> MKKEVRKVRIALASPEKIRSWSYGEVEKPETINYRTLKPERDGLFDERIFGPIKDYECACGKYKRQRFEGKVCERCGVEVTRSIVRRYRMGHIELATPAAHIWFVKDVPSKIGTLLDLSATELEQVLYFNKYIVLDPKGAVLDGVPVEKRQLLTDEEYRELRYGKQETYPLPAGVDALVKDGEEVVKGQELAPGVVSRMDGVALYRFPRRVRVDYLRKERAALRIPLSAWVEKEAYRPGEVLAELSEPYLFRAEESGVVELKDLAEGHLIYLRQEEEVVARYFLPAGMTPLVVEGEIVEVGQPLAEGKGLLRLPRHMTAKEVEAEEEGDSVHLTLFLEWTEPKDYKVAPHMNVIVPEGAKVQAGEKIVAAIDPEEEVIAEAEGVVHLHEPASILVVKARVYPFEDDVEVTTGDRVAPGDVLADGGKVKSEIYGRVEVDLVRNVVRVVESYDIDARMGAEAIQELLKELDLEKLERELLEEMKHPSRARRAKARKRLEVVRAFLDSGNRPEWMILEAVPVLPPDLRPMVQVDGGRFATSDLNDLYRRLINRNNRLKKLLAQGAPEIIIRNEKRMLQEAVDAVIDNGRRGSPVTNPGSERPLRSLTDILSGKQGRFRQNLLGKRVDYSGRSVIVVGPQLKLHQCGLPKRMALELFKPFLLKKMEEKAIAPNVKAARRMLERQRDIKDEVWDALEEVIHGKVVLLNRAPTLHRLGIQAFQPVLVEGQSIQLHPLVCEAFNADFDGDQMAVHVPLSSFAQAEARIQMLSAHNLLSPASGEPLAKPSRDIILGLYYITQVRKEKKGAGMAFATPEEALAAYERGEVALNAPIVVAGRETSVGRLKFVFANPDEALLAVAHGLLDLQDVVTVRYLGRRLETSPGRILFARIVGEAVGDEKVAQELIQMDVPQEKNSLKDLVYQAFLRLGMEKTARLLDALKYYGFTLSTTSGITIGIDDAVIPEEKQRYLEEADRKLRQIEQAYEMGFLTD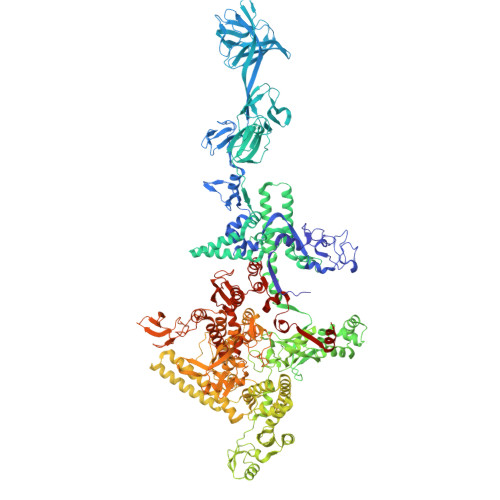RERYDQVIQLWTETTEKVTQAVFKNFEENYPFNPLYVMAQSGARGNPQQIRQLCGMRGLMQKPSGETFEVPVRSSFREGLTVLEYFISSHGARKGGADTALRTADSGYLTRKLVDVAHEIVVREADCGTTNYISVPLFQMDEVTRTLRLRKRSDIESGLYGRVLAREVEALGRRLEEGRYLSLEDVHFLIKAAEAGEVREVPVRSPLTCQTRYGVCQKCYGYDLSMARPVSIGEAVGVVAAESIGEPGTQLTMRTFHTGGVAVGTDITQGLPRVIELFEARRPKAKAVISEIDGVVRIEEGEDRLSVFVESEGFSKEYKLPKDARLLVKDGDYVEAGQPLTRGAIDPHQLLEAKGPEAVERYLVDEIQKVYRAQGVKLHDKHIEIVVRQMLKYVEVTDPGDSRLLEGQVLEKWDVEALNERLIAEGKVPVAWKPLLMGVTKSALSTKSWLSAASFQNTTHVLTEAAIAGKKDELIGLKENVILGRLIPAGTGSDFVRFTQVVDQRTLKAIEEARKEAVEAKEKEAPRRPVRREQPGKGL Plicamycin, mithramycin analogue MTM SA-Trp | C61 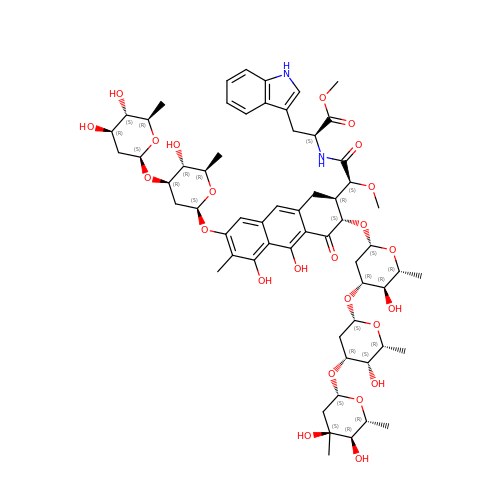H82 N2 O24 | HDFPUIGVWMMVMM-CPYVCCANSA-N> MSVETPSALADSSPHTAPGSAGRSLELGAADIQDLESFEAGRGALPARAYLQSDAPRLSLNGEWQFRLSPGSRVAPDDGWQLGEALNGFESLPVPSSWPMHGHGAPAYTNVQFPFAVEPPHVPEANPIGDHLVVFEAGPEFFPHALLRFDGIESAGTVWLNGVELGTTRGSRLAHEFDVSGILEQGENTLAVRVAQFSAASYVEDQDMWWLPGIFRDVTLQARPAAGIDDVFVHAGYDHITGEGILKVEASRGGQAIDAVVRVPELALELAAGTEVRVPAVEPWSAEVPKLYEAAVSAAGESVALQIGFRSIAIEDAQFKVNGRRILLRGVNRHEHHPRLGRVVPRDVVEAELRLMKQHNINAIRTSHYPPHPQFLALADQLGFYVVLECDLETHGFESAGWAQNPSDDPQWEDALVDRMRRTVERDKNHASVVMWSLGNEAGTGRNLAAMSRWTKDRDPSRPIHYEGDWSSEHVDVYSRMYASQAETALIGQGIEPALNDAALDARRRAMPFVLCEYVHAMGNGPGGMSEYQALFEKYPRLMGGFVWEWLEHGITVSTADGVDHYGYGGDFGEEVHDGNFVTDGLVDADRRPRPGLLDFKKVIEPLRIDVARDWTGFTLRNGQDFADTSAFSFRYEVEADGGALDGGTVDVAPVAPQSETVVELPGSVAALAAGLSDGRPAVLTVRAVLGADSAWADAGHEVAWGQSVREPGAPVPPAPVEPVQVQDSELTLGPVVFSRATGMPTSIGGVPVEKLGLTLWWAPTDNDLGREWGGADERPLATQWKDAGLNRLHTRLLGISANPGQDGGETLTVRTRVSAADKQYGVLVDYTWSTDGETVGLRTQVRRDGTWVNRGFEVEWARIGLEFVLGEETELVSWFGQGPHQSYPDTGQGARAGWFSLPLAKMDVEYVRPQECGARSGSRSAALQLGGRTLEICGDPFALTVRPYSQDVLDAAAHRPDLKADGRTYLYVDHALRGVGTAACGPGVLEQYRLKPRDADFILTLKVRS

ArthβDG is a five-domain protein of molecular weight 110 kDa. The catalytic domain, in form of TIM barrel, is surrounded by three IG-like domains and, as typical for the GH2 family, an N-terminal super β-sandwich domain. Regardless of low sequence identity, this monomer’s architecture is strikingly similar to KlyvβDG and EcolβDG, which enabled determination of catalytic residues E441 and E517. Cold-adapted ArthβDG possesses a functional dimer (not typical for the GH2 family).

Usage of native protein would limit us to analysis of substrate binding using substrate analogs which could not by hydrolyzed by the enzyme, such as isopropyl β-d-1-thiogalactopyranoside (IPTG), or less preferable substrates such as ortho-nitrophenyl-β-galactoside (ONPG). Determined crystal structures of ArthβDG complexes with specific ligands may be divided into three groups: complexes with substrates and their analogues (early complexes) ArthβDG_E441Q/LACs, ArthβDG/IPTG; the second group are intermediates complexes ArthβDG_E441Q/LACd ArthβDG/ONPG; and the third one is the complex with product ArthβDG/GAL. The early complexes with substrate show LAC and IPTG binding in shallow mode, intermediate complexes depicts deep binding of substrate that directly precedes formation of galactosyl-enzyme covalent bond, and the product complex allows description of the product release process. At the early stage of the reaction, the substrate is bound in the shallow binding site where the galactosyl group is stabilized by a number of H-bonds between its hydroxyl groups and residues N110, E441, E517, M481, H520, and H368 via water molecules and by an interaction with a sodium ion. On the other hand, the glucosyl moiety of lactose, or the non-galactose moieties of IPTG and ONPG, are hardly stabilized by any interactions during shallow binding.Rv0864 (MoaC2) from Mycobacterium tuberculosis is one of the enzymes in the molybdenum cofactor (Moco) biosynthesis pathway. Together with MoaA, MoaC is involved in the conversion of guanosine triphosphate (GTP) to precursor Z, the first step in Moco synthesis. The MoaC2 monomer has a common α+β protein fold that is composed of a four stranded anti-parallel β-sheet and three helices, α1, α 2 and α3 located underneath the β-sheet. The fold of MoaC belongs to the ferredoxin like family (βαββαβ) with one additional helix (βααββαβ) not typically present in a prototypical ferredoxin-like molecule.

The crystal structure of the Moco-biosynthesis protein MoaC2 (Rv0864) in its apo form from Mycobacterium tuberculosis has been determined to 2.2 Å. The asymmetric unit of Rv0864 (MoaC2) contains a dimer and three such dimers related by crystallographic symmetry associate to form a hexamer, which is the biological assembly. The two independent subunits in the structure superpose onto each other with a root mean square deviation (r.m.s.d) of 0.35 Å for 120 Cα atoms. Closer examination of the superposition reveals conformational differences in the additional helix α1, wherein the r.m.s.d between α1 region of subunit A and B is 0.46 Å. Upon dimerization, the 4-stranded anti parallel beta sheets of both monomers associate to form a contiguous 8 stranded sheet. The α3 helix is present at the dimer interface of MoaC2, α2 helix, loop region residues 83–89 (LIPLCHQ) and Leu122 and Ile148 are mainly involved in the dimerization of the protein molecule. Lys78 which is conserved in all MoaC proteins is located in the α2 helix of the adjacent dimer forms three strong hydrogen bonds through its NZ (Average distance 2.8 Å) to the main chain carbonyl group of residues Ser81, Pro85 and Cys87, with an average distance of ∼2.8 Å resulting in an approximately three fold symmetrical arrangement. The α1 helix 48–57, which is not typically present in the ferredoxin fold, shows a higher deviation when superposed with the other existing reported structures and it is not typically present in ferredoxin like fold. This helix lies adjacent to the ligand binding site and may impart functional role. In fact, one of the native crystals soaked in 10 mM GTP diffracted to 2.8 Å, but no GTP could be seen in the electron density map (Data not shown).

>[2x]MARASGASDYRSGELSHQDERGAAHMVDITEKATTKRTAVAAGILRTSAQVVALISTGGLPKGDALATARVAGIMAAKRTSDLIPLCHQLALTGVDVDFTVGQLDIEITATVRSTDRTGVEMEALTAVSVAALTLYDMIKAVDPGALIDDIRVLHKEGGRRGTWTRRLEHHHHHH>[4x]GSGSVQATDRLMKELRDIYRSQSFKGGNYAVELVNDSLYDWNVKLLKVDQDSALHNDLQILKEKEGADFILLNFSFKDNFPFDPPFVRVVSPVLSGGYVLGGGAICMELLTK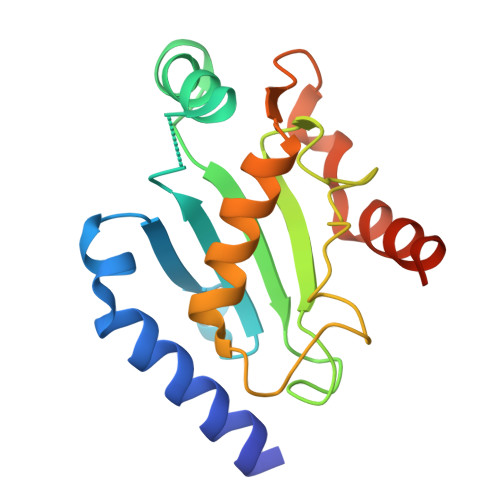QGWSSAYSIESVIMQISATLVKGKARVQFGANKSQYSLTRAQQSYKSLVQIHEKNGW> MTKKTEIPSHLKPFVSTQHYDQYTPVNHAVWRYIMRQNHSFLKDVAHPAYVNGLQSSGINIDAIPKVEEMNECLAPSGWGAVTIDGLIPGVAFFDFQGHGLLPIATDIRKVENIEYTPAPDIVHEAAGHAPILLDPTYAKYVKRFGQIGAKAFSTKEEHDAFEAVRTLTIVKESPTSTPDEVKAAENAVIEKQNLVSGLSEAEQISRLFWWTVEYGLIGNIDDPKIYGAGLLSSVGESKHCLTDAVEKVPFSIEACIGTTYDVTKMQPQLFVCESFEELTDALETFSKTMAFKTGGKEGLEKAIRSENYATAELNSGLQITGTFSETIENDAGELIYMRTNSPTALALHNKQLANHSTSVHSDGFGTPIGLLTENIALENCTDEQLQSLGITIGTIAEFTFASGIHVKGTVTDIVKNDKKIALISFIDCTVTYNARVLFDASWGAFDMAVGSQITSVFPGAADAAAFFPMDEEVHEIPA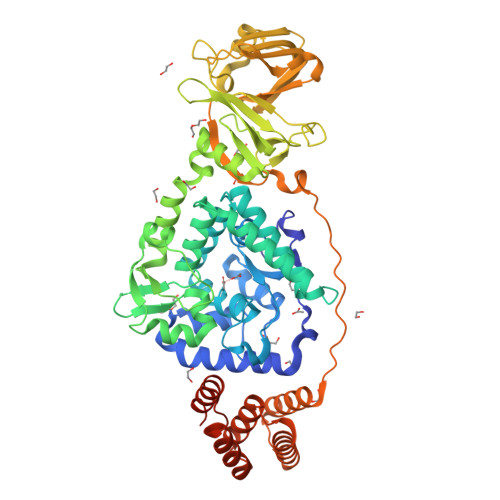PLVLNELERMYQTVRDIRSEGILHDAHIDQLIAIQEVLNKFYAKEWLLRLEVLELLLEHNKGHETSAALLHQLSTFTTDEAVTRLINNGLALLPVKDVKNDAKINLEHHHHHH> PISPIETVPVKLKPGMDGPKVKQWPLTEEKIKALVEICTEMEKEGKISKIGPENPYNTPVFAIKKKDSTKWRKLVDFRELNKRTQDFWEVQLGIPHPAGLKKKKSATVLDVGDAYFSVPLDEDFRKYTAFTIPSINNETPGIRYQYNVLPQGWKGSPAIFQSSMTKILEPFRKQNPDIVICQYMDDLYVGSDLEIGQHRTKIEELRQHLLRWGLTTPDKKHQKEPPFLWMGYELHPDKWTVQPIVLPEKDSWTVNDIQKLVGKLNWASQIYPGIKVRQLCKLLRGTKALTEVIPLTEEAELELAENREILKEPVHGVYYDPSKDLIAEIQKQGQGQWTYQIYQEPFKNLKTGKYARMRGAHTNDVKQLTEAVQKITTESIVIWGKTPKFKLPIQKETWETWWTEYWQATWIPEWEFVNTPPLVKLWYQLEKEPIVGAETFYVDGAANRETKLGKAGYVTNRGRQKVVTLTDTTNQKTELQAIYLALQDSGLEVNIVTDS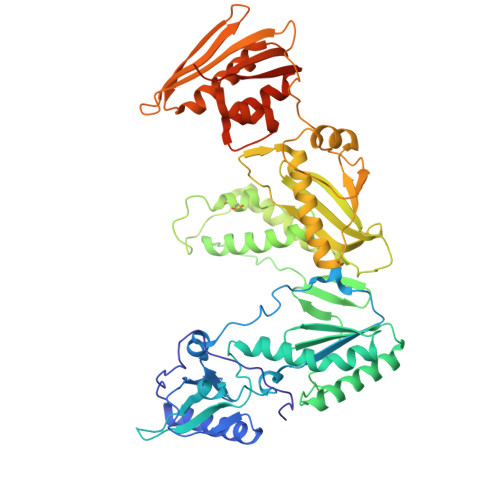QYALGIIQAQPDQSESELVNQIIEQLIKKEKVYLAWVPAHKGIGGNEQVDKLVSAGIRKVL N-DODECANOYL-L-TYROSINE 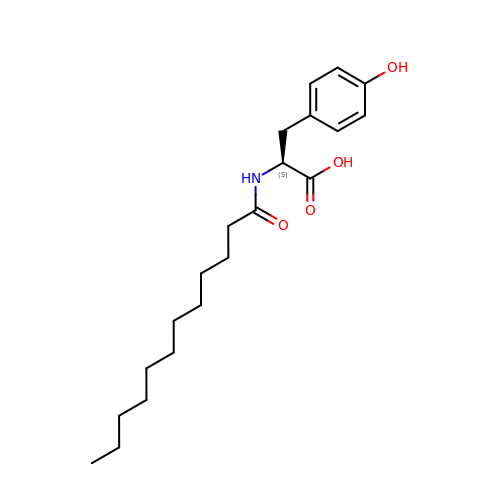| C21 H33 N O4 | SVQAZCRYIXURJT-IBGZPJMESA-N>MHHHHHHHHHHGENLYFQGSDNIISFDHVTFTYPDSPRPALSDLSFAIERGSWTALIGHNGSGKSTVSKLINGLLAPDDLDKSSITVDGVKLGADTVWEVREKVGIVFQNPDNQFVGATVSDDVAFGLENRAVPRPEMLKIVAQAVADVGMADYADSEPSNLSGGQKQRVAIAGILAVKPQVIILDESTSMLDPEGKEQILDLVRKIKEDNNLTVISITHDLEEAAGADQVLVLDDGQLLDQGKPEEIFPKVEMLKRIGLDIPFVYRLKQLLKERGIVLPDEIDDDEKLVQSLWQLNSKM[2x];>MAIKFENVSYVYSPGSPLEAIGLDQLNFSLEEGKFIALVGHTGSGKSTLMQHFNALLKPTSGKIEIAGYTITPETGNKGLKDLRRKVSLAFQFSEAQLFENTVLKDVEYGPRNFGFSEDEAREAALKWLKKVGLKDDLIEHSPFDLSGGQMRRVALAGVLAYEPEIICLDEPAAGLDPMGRLEMMQLFKDYQAAGHTVILVTHNMDDVADYADDVLALEHGRLIKHASPKEVFKDSEWLQKHHLAEPRSARFAAKLEAAGLKLPGQPLTMPELADAIKQSLKGGEHE[2x];>MKSESKVSSKLELRELVLLAMVIAIKVILGQFKVGNATLQVGLGFIGSVMLGYLFGPWWGFAGGALSDLVSSVIFGNLGGFFIGFTLTAALGPMIYGFFLYKQPIQIWRVIASVICVTVICNIGLNTLWVSMMYGINFMVALSSRILKEMITPWIQMVAVWFILEGLSRVKLSRKFWSHPQFEK[2x];>[2x]MSKIIIGRYLPGTTFVYRVDPRAKLLTTFYFIIMIFLANNWVSYLVISIFGLAYVFATGLKARVFWDGVKPMIWMIVFTSLLQTFFMAGGKVYWHWWIFTLSSEGLINGLYVFIRFAMIILVSTVMTVTTKPLEIADAMEWMLTPLKLFKVNVGMISLVISIALRFVPTLFDQTVKIMNAQRSRGADFNDGGLVKRAKSVVPMLVPLFIDSLEVALDLSTAMESRGYKGSEGRTRYRILEWSKVDLIPVAYCLLLTILMITTRKH

ECF transporters consist of two identical or highly similar cytoplasmic ATPases, EcfA and EcfA′, and two transmembrane subunits, EcfT and the S-component124. The membrane-embedded S-component serves as both the substrate-binding and the substrate-translocation domain. The other three subunits (EcfA, EcfA′ and EcfT) together form the ECF module that energizes substrate transport by the S-component456. Here we report crystal structures of the group II ECF transporter for folate from Lactobacillus delbrueckii (L. delbrueckii) in the apo-state and in complex with the slowly hydrolysable ATP analogue AMP–PNP.

We determined crystal structures of the ECF–FolT2 complex from L. delbrueckii in the apo state (no nucleotides or folate) and in an AMP–PNP-bound state at 3.0 and 3.3 Å resolution, respectively. In both structures of ECF–FolT2, the ATPases EcfA and EcfA′ are in an open conformation with the subunits separated thus leaving the two ATP hydrolysis sites incomplete. The FolT2 proteins in the AMP–PNP-bound and apo complexes do not have folate bound. Nonetheless, the structure of substrate-free FolT2 is very similar to the structure of solitary, folate-bound FolT1 with root mean squared deviation values of 1.35 Å (FolT1 compared with FolT2 from the AMP–PNP-bound structure) and 1.25 Å (FolT1 compared with FolT2 from the apo structure). Although the structures of the apo and AMP–PNP-bound complexes are very similar overall, the relative orientation of the transmembrane and coupling domain of EcfT is different. The coupling domains of the two complexes are in identical positions relative to the two ATPases and FolT. In contrast, the transmembrane domains are in different orientations. In the AMP–PNP structure it is packed tightly against the FolT subunit and interacts with the loops L3 and the C terminus of H5, but in the apo structure it has hinged away and the two membrane proteins interact less tightly. The position of the L1 loop in the complexes is stabilized by a hydrogen bond between the backbone carbonyl group of G35 and the highly conserved R196 (the AMP–PNP structure) or N189 (in the apo structure) in the coupling domain of EcfT. The structural flexibility of the membrane domain of EcfT also suggests that the interactions with loop L3 and H5 from FolT are relatively weak, in contrast to the strong hydrophobic and van der Waals interactions between the rigid coupling domain of EcfT and FolT.Ribonuclease P (RNase P) is an endoribonuclease that catalyzes the processing of the 5′ leader sequence of precursor tRNA (pre-tRNA). Recently, minimal PRORP (approximately 23 kDa) has been reported in bacteria and archaea. This type was initially found in the hyperthermophilic bacterium Aquifex aeolicus (gene name: aq880). Bioinformatics analysis has shown that homologs of Aq880 are widely present in some phyla of bacteria and archaea (termed HARPs for homologs of Aquifex RNase P).

After 3D classification, the particles converged into a single prominent class with a resolution of 3.62 Å. The cryo-EM structure revealed that Aq880 is a homododecamer. Each subunit has a typical PIN-like fold, which comprises a single α/β/α domain with a five-stranded parallel β-sheet (β1-β5) surrounded by nine α-helices (α1-α9). Notably, each subunit also possesses two prominent helices (α5 and α6) that are inserted into the nuclease domain. Hence, the region of the two helices was denoted as the “protruding helical” (PrH) domain. The two subunits formed a dimer mediated by the PrH domain, consisting of α5 and α6. The dodecameric assembly of Aq880 showed a left-handed one-turn superhelical structure with six dimers. Each dimer was aligned side-by-side with β-sheet interactions to form a hexamer of the dimer. In the present study, the structure of Aq880 revealed that these aspartate residues are localized in the nuclease domain near the PrH domain, representing the active site of Aq880. The structure of Aq880 revealed that the active site of Aq880 contains five acidic residues required for catalysis, which is analogous to the active site of eukaryotic PRORPs.

>ATSMDVFVLDTSVFTNPEIYRTFEEDQRGAMETFIHLALNSRAEFYMPTSVYTEMRKIMDVGELWAEFEMVVKIRSPRRFQLTVPADFLYEFIEELRYRINKGLRIAEEHTREASGCEDVGKLIARLREKYREALRQGILDSKEDVDVLLLAYELDGVLVSADEGLRTWADKIGIKLIDPKNFKNILESLVRHRF[12x]>MKDLKGTKTAENLKQGFIGESMANRRYLYFAKRADEEGYPEIAGLLRSIAEGETAHAFGHLDFIRQGGLTDPATDKPIGTLEQMIESAIAGETYEWTQMYPGFAKVAREEGFPEVAEWFETLARAEKSHA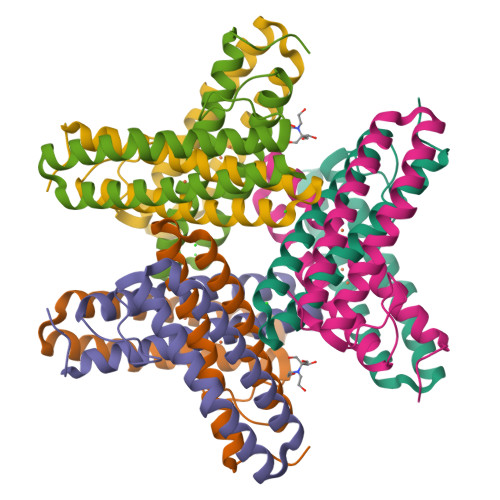EKFQNVLKQLKGGT[3x]> MAGTSFLSDLLSGVTERGRALLFSGSKARDRVVDTDIETLCEMLLSSRGEASGMAIAAEILDRWSRFNAAEAVQFLHMLSDRFGAEAAALDKAIDAYRTDKSPMAVIALHNAAEPRRQELLRRLNLAPNGTQKLVRMRERLLETKEDRADLGAVDTDFAHLFSSWFNRGFLTLQPIDWTTPAHILEK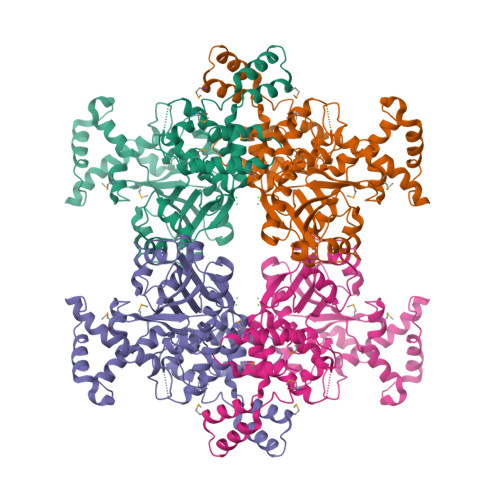IIKYEAVHEIAGWEELRRRLAPADRRCFAFFHPRLRDDPLVFVEVALTRSIPSAIADVLDESRDHIGADTATTAVFYSISNCQDGLRGISFGNFLIKQVVEDLRRDLPGLKEFVTLSPVPGFARWISKIRDPKSGFPLSPEDRNTLVLLDDPTWPEDKARADAVERILLPLAARYFITERTPDNRPVDPVARFHLGNGARLERLNFLGDRSVKAMRQAHGLMVNYLYKLEDIETNHEALAQRGEVAASPAVKALQGKIEPILEHHHHHH> SREQIIKDGGNILVTAGAGSGKTTILVSKIEADLKENKTHYSIAAVTFTNKAAKEIEGRLGYSSRGNFIGTNDGFVESEIIRPFIKDAFGNDYPDNFTAEYFDNQFASYDKGLQVLKYQNILGTYSNPKKNFKFQLALDILKKSLVARQYIFSKYFKIFIDEYQDSDKDMH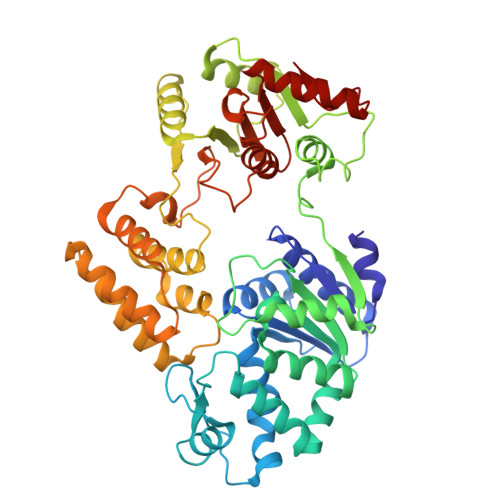NLFMYLKDQLKIKLFIVGDPKQSIYIWRGAEPENFNGLIENSTDFNKYHLTSNFRCCQDIQNYSNLFNEETRSLIKEKNEVQNVISIADDMPISDILLKLTEEKQVLNIEAELVILVRRRNQAIEIMKELNEEGFNFIFIPQTPLDRATPNATLLKEVIKYVKNDRYSIYDLAAEIVGNLSSREIKEIQKIINELLVPNINQVLINQVLINLFAKLEITLDTREITAFTEVMMTNEFDIAFDTNEYLHKIFTVHSAKGLEFNQVIITASDYNVHYNRDTNEHYVATTRAKDKLIVIMDNKKYSDYIETLMKELKIKNIIKSI>GSQDSTSDLIPAPPLSKVPLQQNFQDNQFQGKWYVVGLAGNAILREDKDPQKMYATIYELKEDKSYNVTSVLFRKKKCDYWIRTFVPGSQPGEFTLGNIKSYPGLTSYLVRVVSTNYNQHAMVFFKKVSQNREYFKITLYGRTKELTSELKENFIRFSKSLGLPEN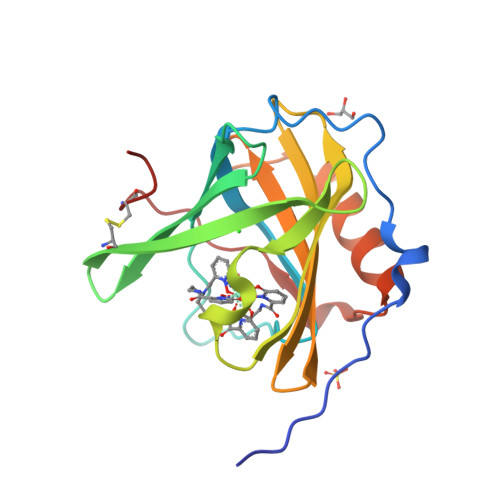HIVFPVPIDQCIDG[6x]> SIWSRVVQFGTGWGFWVSGHVFITAKHVAPPKGTEIFGRKPGDFTVTSSGDFLKYYFTSAVRPDIPAMVLENGCQEGVVASVLVKRASGEMLALAVRMGSQAAIKIGSAVVHGQTGML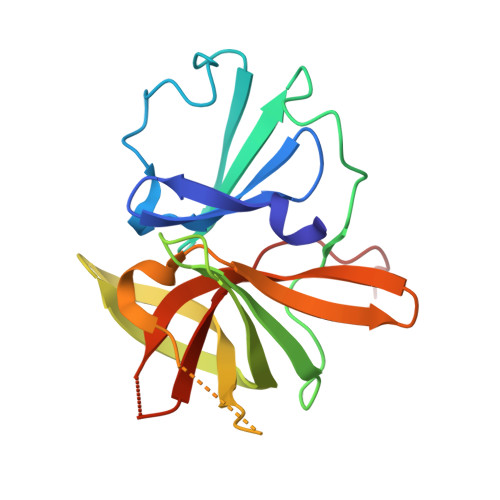LTGSNAKAQDLGTIPGDAGCPYVYKKGNTWVVIGVHVAATRSGNTVIAATHGEPTLEA> MDTLEGSMAQLKKGLESGTVLIQFEQLYRKKPGLAITFAKLPQNLDKNRYKDVLPYDTTRVLLQGNEDYINASYVNMEIPAANLVNKYIATQGPLPHTCAQFWQVVWDQKLSLIVMLTTLTERGRTKCHQYWPDPPDVMNHGGFHIQCQSEDCTIAYVSREMLVTNTQTGEEHTVTHLQYVAWPDHGVPDDSSDFLEFVNYVRSLRVDSEPVLVHCSAGIGRTGVLVTMETAMCLTERNLPIYPLDIVRKMRDQRAMMVQTSSQYKFVCEAILRVYEEGLVQMLDPS

Protein tyrosine phosphatases (PTPs) play a critical role in regulating cellular functions by selectively dephosphorylating their substrates. The ∼280 residue PTP catalytic domain consists of an α/β structure, and biochemical and structural studies have led to a detailed understanding of the catalytic mechanism (Barford et al., 1994; Zhang, 2002). Key features of the domain include the PTP signature motif, the mobile Trp-Pro-Asp “WPD” loop that in the closed conformation positions the conserved and catalytically important aspartate residue, and the phosphotyrosine recognition loop. Here we report the crystal structures of 22 PTP domains, including two tandem-domain RPTP structures and a detailed structural comparison of this protein family.

In the fourth category, both the gateway and secondary pocket are blocked and the inaccessible binding cavity harbors an aromatic residue or a proline in position of Arg24. The second-site loop assumes a twisted conformation in these phosphatases. This architecture is present in the subgroups NT5 (PTPH1, MEG1), NT6 (PTPD1, PTPD2), R1 (CD45), R2B (RPTPμ, RPTPκ, RPTPρ), and R4 (RPTPα, RPTPɛ). PTPs with particularly high enzymatic activity against generic substrates were RPTPσ and PTP subgroups R5, R3, NT1, NT2, NT3, NT4, and NT5. The subgroups NT1, NT2, NT3, and NT5 exhibited a pronounced preference for acidic residues N-terminal to the phosphorylation site.>MRGSHHHHHHGSMDRAAQIKQIADSWNTPRFAGIVRPYTPEDVYRLRGSVQIEYTLARMGAERLWNLLHTEPYINALGALTGNQAMQQVKAGLKAIYLSGWQVAADANLAGQMYPDQSLYPANSGPQLVRNINNALRRADQIYHSEGRNDIYWFAPIVADAEAGFGGPLNVFEIMKAYIEAGAAGVHFEDQLASEKKCGHMGGKVLIPTQAAIRNLVAARLAADVMGVPTIIVARTDANAATLLTSDIDERDRPFCTGERTSEGFYRVRAGLDQAIARGLAYAPYADMIWCETSEPNLEEARRFAEAIHAQFPGKLLAYNCSPSFNWKKKLDDATIAAFQRELGAMGYKFQFVTLAGFHALNYSMFELARNYRDRGMAAYSELQQAEFAAEAYGYTATRHQREVGTGYFDEVAQVIAGGEISTTA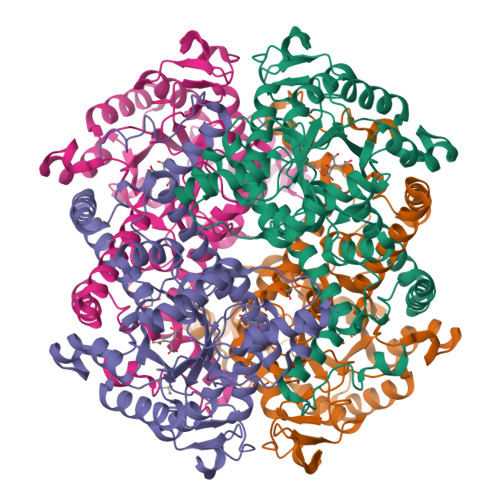LTGSTEEEQFH[8x]>[2x]SNAHSDTAILFSAESEWATRSQTLPSMKLNHWHDVRDWYRAFLDAGSRADIVPLAYDWSSYKTVVLPTVLILSAADTQRLADFAAAGGRVVVGYATGLIDEHFHTW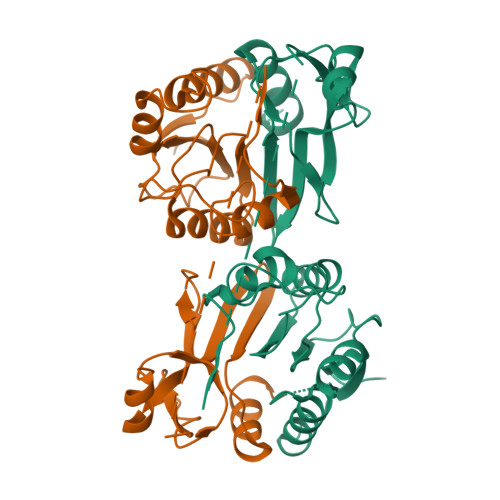LGGYPGAGDGLLRSMLGVRGEEFNILGAEAEGEPGEIRLSSADDSAALDGTTTRLWQNDVNVTGEHAQVLATYAGEEADEWELDGTAAVTRNPYGSGEAYFVGCDLDVADLTKLVRAYLAASSQEN>[2x]EKAKRAVRGRQDRPKEFPPPRYNYTILTRYNATALASPFINDQVKNVDLRIVTATRPCEMIALIAKTNIDSILKELAAAQKTYSARLTWFKIMPTCATPIHDVSYMKCNPKLSFAMCDERSDILWQASLITMAA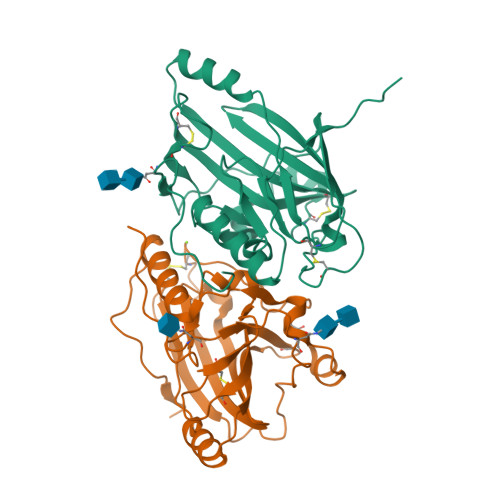ETDDELGLVLAAPAHSASGLYRRVIEIDGRRIYTDFSVTIPSERCPIAFEQNFGNPDRCKTPEQYSRGEVFTRRFLGEFNFPQGEHMTWLKFWFVYDGGNLPVQFYEAQAFARPVPPDNHPGFDSVESEITQNKTDPKPGQADPKPNQPFKWPSIKHLAPRLDEVDEVIEPVTKPPKTSKSNSTFENLYFQGHHHHHH>[2x]GSICQFKLVLLGESAVGK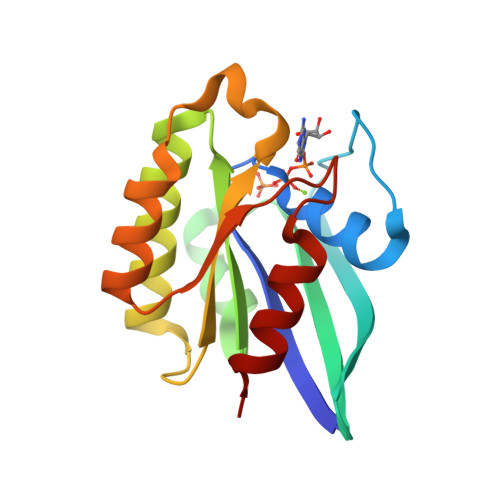SSLVLRFVKGQFHEYQESTIGAAFLTQTVCLDDTTVKFEIWDTAGLERYHSLAPMYYRGAQAAIVVYDITNTDTFARAKNWVKELQRQASPNIVIALAGNKADLASKRAVEFQEAQAYADDNSLLFMETSAKTAMNVNEIFMAIAKKLP> MQRFGTGSSRSWCGRAGTATIAAVLLASGALTGLPPAYAISPPTIDPGALPPDGPPGPLAPMKQNAYCTEVGVLPGTDFQLQPKYMEMLNLNEAWQFGRGDGVKVAVIDTGVTPHPRLPRLIPGGDYVMAGGDGLSDCDAHGTLVASMIAAVPANGAVPLPSVPRRPVTIPTTETPPPPQTVTLSPVPPQTV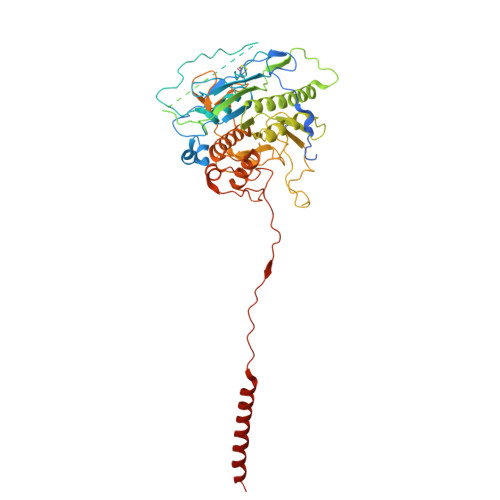TVIPAPPPEEGVPPGAPVPGPEPPPAPGPQPPAVDRGGGTVTVPSYSGGRKIAPIDNPRNPHPSAPSPALGPPPDAFSGIAPGVEIISIRQSSQAFGLKDPYTGDEDPQTAQKIDNVETMARAIVHAANMGASVINISDVMCMSARNVIDQRALGAAVHYAAVDKDAVIVAAAGDGSKKDCKQNPIFDPLQPDDPRAWNAVTTVVTPSWFHDYVLTVGAVDANGQPLSKMSIAGPWVSISAPGTDVVGLSPRDDGLINAIDGPDNSLLVPAGTSFSAAIVSGVAALVRAKFPELSAYQIINRLIHTARPPARGVDNQVGYGVVDPVAALTWDVPKGPAEPPKQLSAPLVVPQPPAPRDMVPIWVAAGGLAGALLIGGAVFGTATLMRRSRKQQ>GMENVITYNNDKGLLAYIQFLASSAQKIGDGNTDRVFDFEDALDQTQMAQLAVDELKKIPEVNALFSERWLPAPFNLDDLAKLPEGTLGHVYAREMKARGFDPYFYKKVPVVDDISYLKMLWRSTHD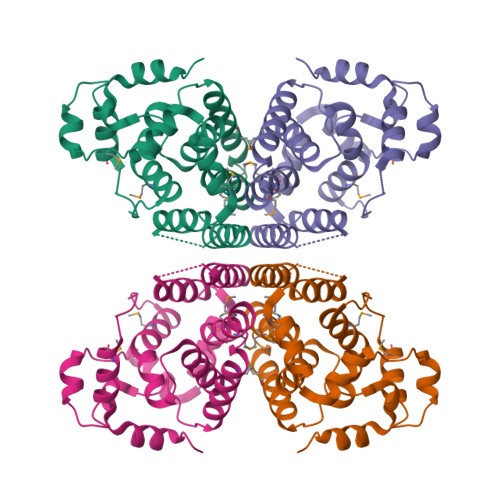IYHVVAGFDTNVFGEIGLQAFFLAQTPIPISVMLLSFGMVMISLYQPTNFKALMTEISRGYRVGSHTPGKLIAQKWDQLWDVQVSEIRERLGVNSIL[4x]> GSGREEDPHEGKIWFHGKISKQEAYNLLMTVGQVSSFLVRPSDNTPGDYSLYFRTNENIQRFKISPTPNNQFMMGGRYYNSIGD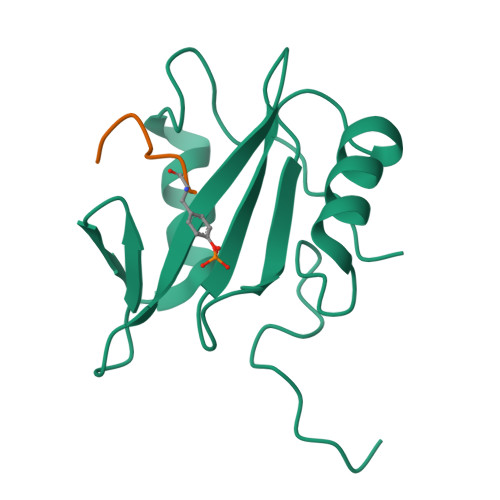IIDHYRKEQIVEGYYLKEPVPMQ;> XDYAEPMDAX Myristoleic acid 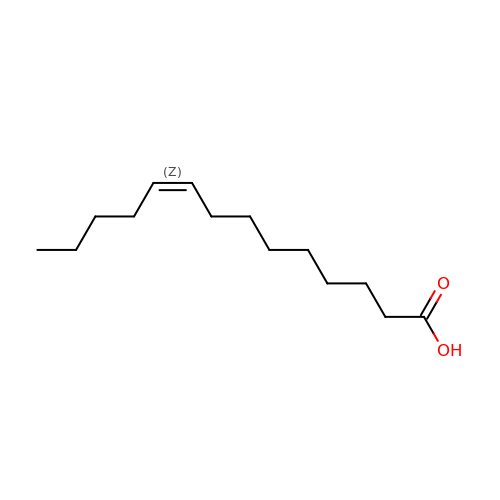| C14 H26 O2 | YWWVWXASSLXJHU-WAYWQWQTSA-N>[2x]VMKANVTKKTLNEGLGLLERVIPSRSSNPLLTALKVETSEGGLTLSGTNLEIDLSCFVPAEVQQPENFVVPAHLFAQIVRNLGGELVELELSGQELSVRSGGSDFKLQTGDIEAYPPLSFPAQADVSLDGGELSRAFSSVRYAASNEAFQAVFRGIKLEHHGESARVVASDGYRVAIRDFPASGDGKNLIIPARSVDELIRVLKDGEARFTYGDGMLTVTTDRVKMNLKLLDGDFPDYERVIPKDIKLQVTLPATALKEAVNRVAVLADKNANNRVEFLVSEGTLRLAAEGDYGRAQDTLSVTQGGTEQAMSLAFNARHVLDALGPIDGDAELLFSGSTSPAIFRAVGGGGGYMAVMVTLRVENLYFQ

The bacterial DNA polymerase III β subunit (β-clamp), and the corresponding eukaryotic and archaeal proliferating cell nuclear antigen (PCNA) are ring-shaped proteins that encircle double-stranded DNA. They act as a processivity factor, or a sliding clamp, for a wide variety of proteins that act on DNA including DNA polymerases, DNA ligase, endonucleases and glycosylases. The structures show that the bacterial sliding clamp is a head-to-tail dimer, where one of the interfaces is opened by the clamp loader to allow DNA to enter the ring interior. In this paper, we describe the crystallographic structure of the DNA polymerase III β-clamp from the extremely radiation resistant bacterium Deinococcus radiodurans (Drβ-clamp).

The crystal structure of Drβ-clamp was determined in space group P3221 to 2.0 Å resolution using molecular replacement. The asymmetric unit contains one Drβ-clamp dimer (residues 1 to 361 of chains A and B), with 292 solvent atoms. Despite our efforts, the DNA oligomer the Drβ-clamp was co-crystallised with was not clearly visible in the electron density, and could not be modelled into the structure. The overall structure of Drβ-clamp is similar to E.coli β-clamp (Ecβ-clamp) and consists of a dimer which forms a ring lined by 12 α-helices, with an opening big enough to accommodate dsDNA. Each monomer consists of three domains (A, B, and C) with identical topology. The shape of the Drβ-clamp dimer is slightly more elliptic than that of the circular Ecβ-clamp, with an internal diameter of 32 to 41 Å. Drβ-clamp displays a strong negative electrostatic surface potential on the outside of the ring, but a more even charge distribution inside the ring on the DNA binding surface and in the dimer forming interface. In E. coli, M. tuberculosis and T. maritima clamps the positive charge forms a relatively continuous band pattern across the surface whereas in Drβ-clamp the charge is more spread forming small positive patches separated by negatively charged areas. The Drβ-clamp dimer interfaces have a spread, even charge distribution compared to the very strong positive (N-terminal domain) and negative charge (C-terminal domain) of the Ecβ-clamp interfaces. In Drβ-clamp these tyrosines are substituted by Ala151 and Val152, which may explain why the DNA is bound in a too disorganised fashion to be clearly visible in the electron density.Roundabout (Robo) receptors provide an essential repulsive cue in neuronal development following Slit ligand binding. The Drosophila and vertebrate Robo1-3 are most similar, containing five immunoglobulin (Ig) and three fibronectin (Fn) domains in their extracellular region. Here we present the crystal structure of Robo1 Ig1-4 and Robo1 Ig5, together with a negative stain electron microscopy reconstruction of the Robo1 ectodomain. These results show how the Robo1 ectodomain is arranged as compact dimers, mainly mediated by the central Ig domains, which can further interact in a “back-to-back” fashion to generate a tetrameric assembly.

The Robo1 Ig1-4 domains are arranged in an extended conformation, ∼170 Å in length, with essentially no polypeptide linker between any of the four domains. We obtained similar Robo1 Ig1-4 crystals in a different crystallization condition with a c axis ∼10 Å longer. Although these diffracted to a higher resolution, the Ig1 domain was disordered. Otherwise the structures are identical, apart from the βC-βD loop region of Ig4, which is better resolved in the higher-resolution dataset. Nevertheless, four crystallographic contact interfaces are observed. The first results in a dimeric arrangement between 2-fold symmetric molecules along the b axis, and is primarily mediated by the Ig4 domain. This interface, which spans residues 378–394 and 429–436, has the largest buried surface (663 Å2 of each molecule's surface area), and is predominantly hydrophobic in nature.

> QEDFPPRIVEHPSDLIVSKGEPATLNCKAEGRPTPTIEWYKGGERVETDKDDPRSHRMLLPSGSLFFLRIVHGRKSRPDEGVYVCVARNYLGEAVSHNASLEVAILRDDFRQNPSDVMVAVGEPAVMECQPPRGHPEPTISWKKDGSPLDDKDERITIRGGKLMITYTRKSDAGKYVCVGTNMVGERESEVAELTVLERPSFVKRPSNLAVTVDDSAEFKCEARGDPVPTVRWRKDDGELPKSRYEIRDDHTLKIRKVTAGDMGSYTCVAENMVGKAEASATLTVQEPPHFVVKPRDQVVALGRTVTFQCEATGNPQPAIFWRREGSQNLLFSYQPPQSSSRFSVSQTGDLTITNVQRSDVGYYICQTLNVAGSIITKAYLEVTD>GPLGSMAQSTVLPMHCLYGIFLEGNLKIQKNDQEGLKKFKDNIKKFTLELDEIDKISPQSRIGGAICFSSDIWDTVTKKISKPKELKSVNTLSSYMPGTSQRDILIHIISDRMDTCFKLAQDTMRNFGEDQLDIKQEIHGFRRVEERDLTDFIDGTENPDGDELRTQYGLVAAGQPNEFGSYVFTQRYVHNLKKWYPEPLSVQQDTVGRTKKDSI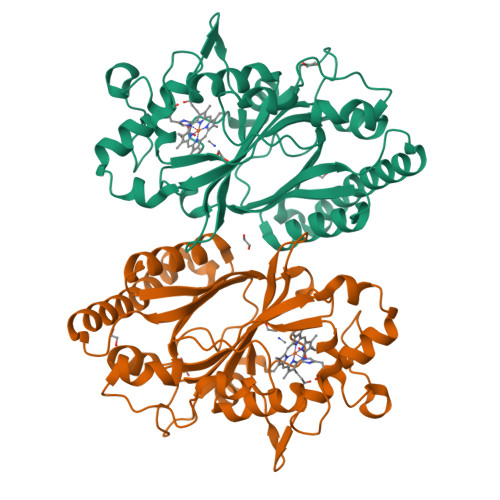EIPRDKRPITSHVSRTDLSENGKDLKIVRQSLPYGQITGEKGLMFIAYACSLHNIEKQLQSMFGQLDGKHDLLLKYTTPVTGSFYFAPSKKELLEL[2x]>[2x]MALSDRLELVSASEIRKLFDIAAGMKDVISLGIGEPDFDTPQHIKEYAKEALDKGLTHYGPNIGLLELREAIAEKLKKQNGIEADPKTEIMVLLGANQAFLMGLSAFLKDGEEVLIPTPAFVSYAPAVILAGGKPVEVPTYEEDEFRLNVDELKK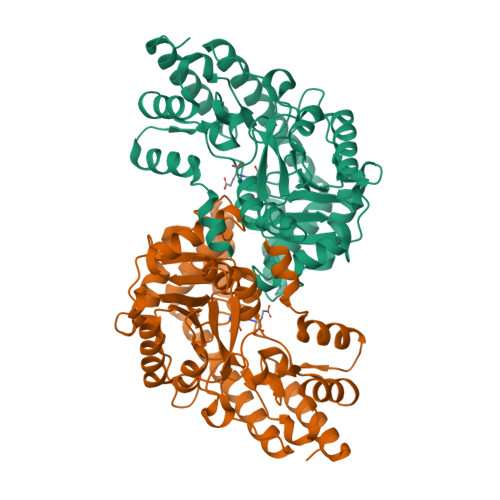YVTDKTRALIINSPCNPTGAVLTKKDLEEIADFVVEHDLIVISDEVYEHFIYDDARHYSIASLDGMFERTITVNGFSKTFAMTGWRLGFVAAPSWIIERMVKFQMYNATCPVTFIQYAAAKALKDERSWKAVEEMRKEYDRRRKLVWKRLNEMGLPTVKPKGAFYIFPRIRDTGLTSKKFSELMLKEARVAVVPGSAFGKAGEGYVRISYATAYEKLEEAMDRMERVLKERKLV> MVAVEQSEASRLGPVFDSCRANNRAALIGYLPTGYPDVPASVAAMTALVESGCDIIEVGVPYSDPGMDGPTIARATEAALRGGVRVRDTLAAVEAISIAGGRAVVMTYWNPVLRYGVDAFARDLAAAGGLGLITPDLIPDEAQQWLAASEEHRLDRIFLVAPSSTPERLAATVEASRGFVYAASTMGVTGARDAVSQAAPELVGRVKAVSDIPVGVGLGVRSRAQAAQIAQYADGVIVGSALVTALTEGLPRLRALTGELAAGVRLGMS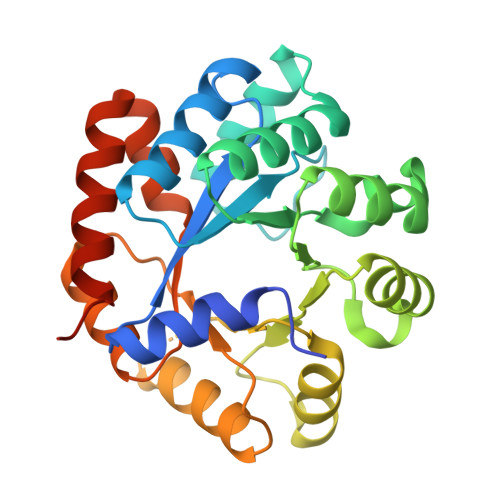AHHHHHH> MGRKRLIT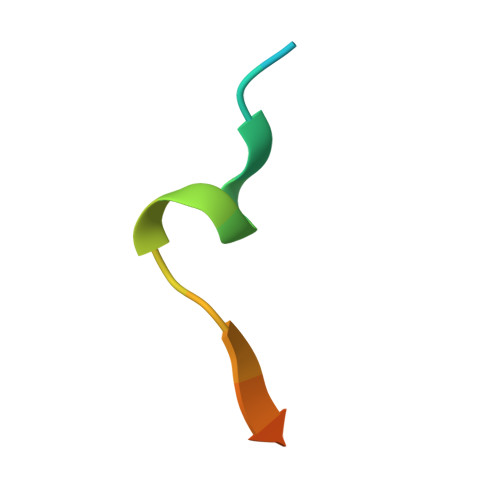DSYPVVKRREG>[2x]SNAAKPLPKEMEDFVQSSGENGVVVFSLGSMVSNMTEERANVIAS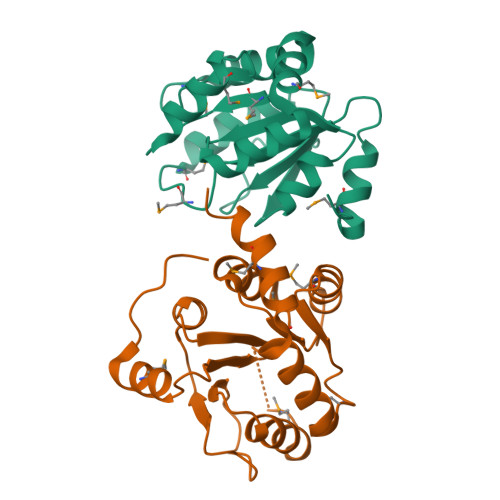ALAQIPQKVLWRFDGNKPDTLGLNTRLYKWIPQNDLLGHPKTRAFITHGGANGIYEAIYHGIPMVGIPLFADQPDNIAHMKARGAAVRVDFNTMSSTDLLNALKRVINDPSYKENVMKLSRIQHD> ASSNLIKQLQERGLVAQVTDEEALAERLAQGPIALVCGFDPTADSLH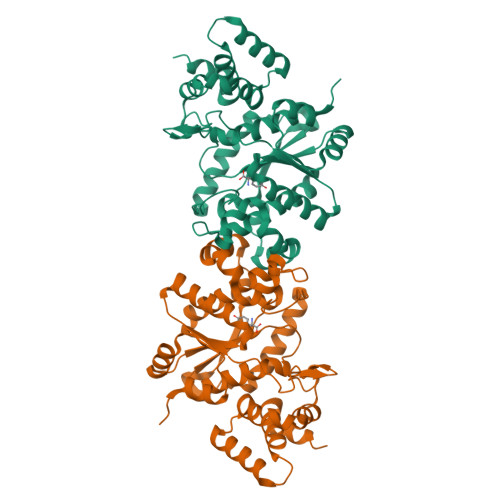LGHLVPLLCLKRFQQAGHKPVALVGGATGLIGDPSFKAAERKLNTEETVQEWVDKIRKQVAPFLDFDCGENSAIAANNYDWFGNMNVLTFLRDIGKHFSVNQMINKEAVKQRLNREDQGISFTEFSYNLLQGYDFACLNKQYGVVLCIGGSDQWGNITSGIDLTRRLHQNQVFGLTVPLITKADGTKFGKTEGGAVWLDPKKTSPYKFYQFWINTADADVYRFLKFFTFMSIEEINALEEEDKNSGKAPRAQYVLAEQVTRLVHGEEGLQAAKR>ASNFTQFVLVDNGGTGDVTVAPSNFANGVAEWISSNSRSQAYKVTCSVRQSSAQNRKYTIKVEVPKVATQTVGGVELPVAAWRSYLNMELTIPIFATNSDCELIVKAMQGLLKDG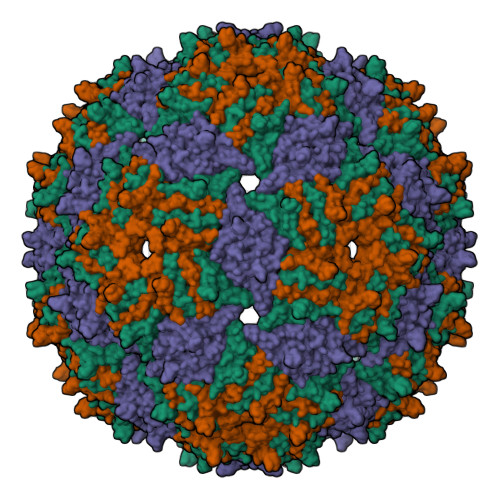NPIPSAIAANSGIY[3x]> GPHLQAPTWYGEPSPAAHWAFGGKLVQITPDGKGVSITNPKISGLESNTTLSEALKTKDFKPLINQRLVKVIDDVNEEDWNLLEKLSMDGTEEFLKEALAFDNDESGNIEQTISKNLVSGNIKSAVKNSLENDLLMEAMVIALDSNNERLKESVKNAYFAKYGSKSSLSRILYSISKREVDDLVENLDVSQWKFISKAIQNLYPNDIAQRNEMLIKLGDRLKENGHRQDSLTLYLAAGSLDKVASIWLSEFPDLEDKLKKDNKTIYEAHSECLTEFIE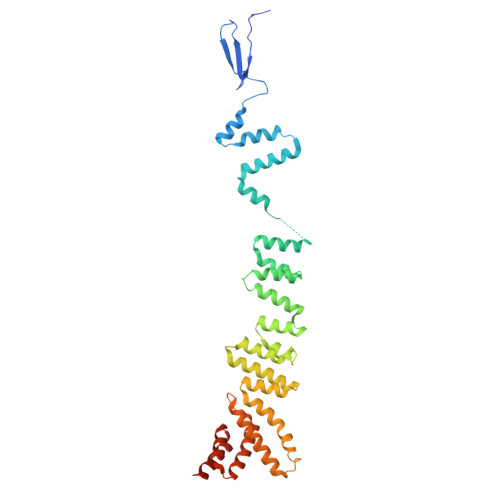RFTVFSNFINGSSTINNEQLIAKFLEFINLTTSTGNFELATEFLNSLPSDNEEVKTEKARVLIASGK>MSLKITKVEVIPISTPMKRAQLMRGATLARIDGVLLKLHSDEGLVGIADAGDTSSWYRGETQDSITSMICDFFAPKVLLGEDPTKIEKIVGRMDILTRDNNQAKATVDFALHDLVGKRFGVPVYQLLGGKTIERIPLGLVLGAGEPEAVAEEALAVLREGFHFVKLKAGGPLKADIAMVAEVRRAVGDDVDLFIDINGAWTYDQALTTIRALEKYNLSKIEQPLPAWDLDGMARLRGKVATPIYADESAQELHDLLAIINKGAADGLMIKTQKAGGLLKAQRWLTLARLANLPVICGCMVGSGLEASPAAHLLAANDWIAQFPQENAGPLHIHDCLNSRDIDNDIALNVPRFEGGYLYPNDGPGLGIELNEDLVRRLVTPGKAARVVTAEGHHHHH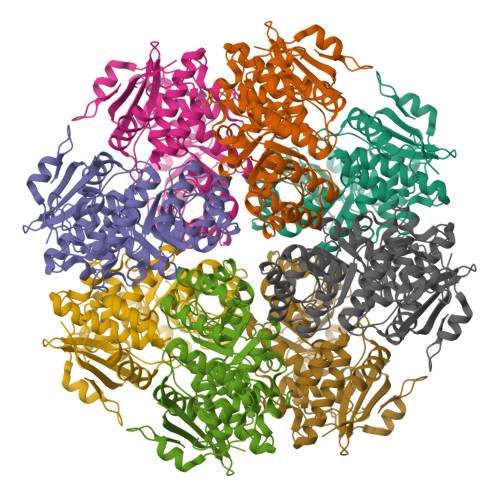H[8x]> VEYRNWSKPQCQITGFAPFSKDNSIRLSAGGDIWVTREPYVSCDPVKCYQFALGQGTTLDNKHSNDTVHDRIPHRTLLMNELGVPFHLGTRQVCIAWSSSSCHDGKAWLHVCITGDDKNATASFIYDGRLVDSIGSWSQNILRTQESECVCINGTCTVVMTDGSASGRADTRILFIEEGKIVHISPLAGSAQHVEECSCYPRYP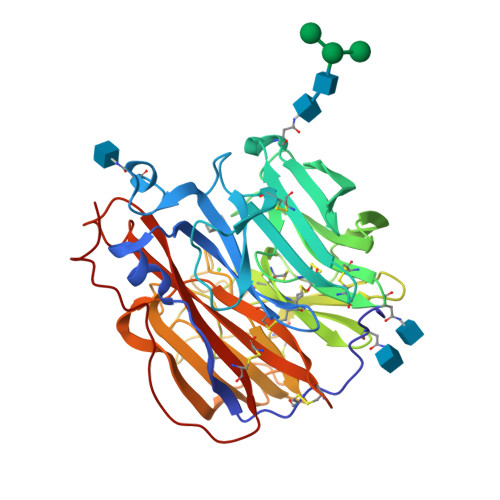GVRCICRDNWKGSNRPVVDINMEDYSIDSSYVCSGLVGDTPRNDDRSSNSNCRDPNNERGTQGVKGWAFDNGNDLWMGRTISKDLRSGYETFKVIGGWSTPNSKSQINRQVIVDSDNRSGYSGIFSVEGKSCINRCFYVELIRGRKQETRVWWTSNSIVVFCGTSGTYGTGSWPDGANINFMPI> MTCNIKNGR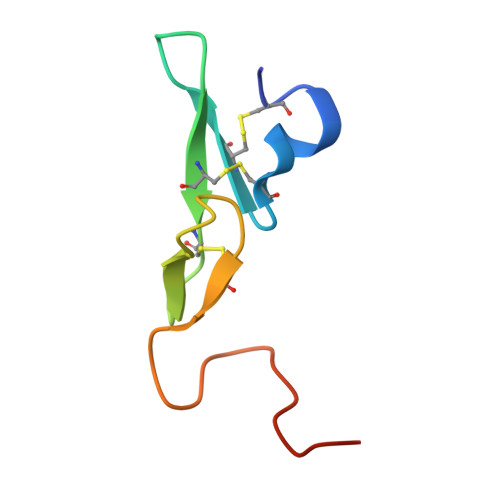CEQFCKNSADNKVVCSCTEGYRLAENQKSCEPAVPFPCGRVSVSQTSK Dipeptidyl peptidase 9 **(**DPP9) is a serine protease cleaving N-terminal dipeptides preferentially post-proline with (patho)physiological roles in the immune system and cancer. On the molecular level, proteases of the DPPIV family are serine aminopeptidases that remove dipeptides from the N-terminus of substrates having a Pro or an Ala residue in the second position (NH_2_-XaaPro/Ala). DPP8 and DPP9 are the only known intracellular members of this family, both localize to the cytosol, the nucleus and associate with the plasma membrane. Here we identify an association of human DPP9 with the tumour suppressor BRCA2, a key player in repair of DNA double-strand breaks that promotes the formation of RAD51 filaments.

We present crystallographic structures documenting the N-terminal Met_1_-Pro_2_ of a BRCA2_1-40_ peptide captured in the DPP9 active-site. A truncated form of the synthetic BRCA2 fragment, lacking the N-terminal residues Met_1_-Pro_2_ (BRCA2_3-40_), bound to DPP9 with lower affinity (KD) of 75.3± 4.8 µM, highlighting the importance of the N-terminal dipeptide Met_1_-Pro_2_ for binding to DPP9 ([Fig fig1]). Previously, we had shown that binding of 1G244 or SLRFLYEG, initiates a rearrangement and a closed conformation of the DPP9 active site. Importantly, the binding of DPP9 to BRCA2_1-40_HA was clearly blocked by SLRFLYEG and 1G244, demonstrating the importance of the open DPP9 active site confirmation for binding to the BRCA2 N-terminus ([Fig fig1]). Control reactions contained no DPP9, or included the DPP9 inhibitor SLRFLYEG. These assays demonstrated processing of BRCA2_1-40_ N-terminal peptide by purified DPP9, leading to removal of the dipeptide Met_1_Pro_2_, with the resulting product (BRCA2_3-40_) having an isoleucine in the neo N-terminus ([Fig fig2], Met_1_Pro_2_↓Ile_3_). To further understand the cleavage event, DPP9 crystals were soaked with the BRCA2_1-40_ peptide. Strikingly, DPP9 crystals exhibited positive electron density at the active site corresponding to the N-terminal Met_1_Pro_2_ di-peptide with the proline residue occupying the S1 subsite. Omit map (Fo-Fc; 3σ) of a BRCA2 peptide soaked in DPP8 crystals (C222_1_) and in DPP9 crystals (P12_1_1). There was no trace of electron density for the rest of the peptide ([Fig fig2] and [Table tbl1]). These structures with the di-peptide captured in the active site clearly document intra-crystalline enzymatic activity of DPP8 and DPP9 resulting in the hydrolysis of the BRCA2_1-40_ N-terminal peptide, and release of the BRCA2_3-40_ peptide.

>[4x]MRKVKKLRLDKENTGSWRSFSLNSEGAERMATTGTPTADRGDAAATDDPAARFQVQKHSWDGLRSIIHGSRKYSGLIVNKAPHDFQFVQKTDESGPHSHRLYYLGMPYGSRENSLLYSEIPKKVRKEALLLLSWKQMLDHFQATPHHGVYSREEELLRERKRLGVFGITSYDFHSESGLFLFQASNSLFHCRDGGKNGFMVSPMKPLEIKTQCSGPRMDPKICPADPAFFSFINNSDLWVANIETGEERRLTFCHQGLSNVLDDPKSAGVATFVIQEEFDRFTGYWWCPTASWEGSEGLKTLRILYEEVDESEVEVIHVPSPALEERKTDSYRYPRTGSKNPKIALKLAEFQTDSQGKIVSTQEKELVQPFSSLFPKVEYIARAGWTRDGKYAWAMFLDRPQQWLQLVLLPPALFIPSTENEEQRLASARAVPRNVQPYVVYEEVTNVWINVHDIFYPFPQSEGEDELCFLRANECKTGFCHLYKVTAVLKSQGYDWSEPFSPGEDEFKCPIKEEIALTSGEWEVLARHGSKIWVNEETKLVYFQGTKDTPLEHHLYVVSYEAAGEIVRLTTPGFSHSCSMSQNFDMFVSHYSSVSTPPCVHVYKLSGPDDDPLHKQPRFWASMMEAASCPPDYVPPEIFHFHTRSDVRLYGMIYKPHALQPGKKHPTVLFVYGGPQVQLVNNSFKGIKYLRLNTLASLGYAVVVIDGRGSCQRGLRFEGALKNQMGQVEIEDQVEGLQFVAEKYGFIDLSRVAIHGWSYGGFLSLMGLIHKPQVFKVAIAGAPVTVWMAYDTGYTERYMDVPENNQHGYEAGSVALHVEKLPNEPNRLLILHGFLDENVHFFHTNFLVSQLIRAGKPYQLQIYPNERHSIRCPESGEHYEVTLLHFLQEYLHHHHHH;>[4x]MP> SNAQENQVHIWAVGGCGGEIGSAFEGEVAKGLHSMTYVDTSRANLRDSTLGDDHIYIFKDAAGRELDGSGKKRDENAELICSQIPGILNKHTPGKFNIVVFSLSGGSGSVAGPALVANLLERGERVVCCIVASFDDERQTINADRTFKGLMAAAEGLKRPVIVSYHMNGENGKSEQDVNLDVQVVISQLCVLFSGENRRLDSADLENFLNHPRVTGLEPTITELNTFMGYEWTKENDSPIAFCTLYPKDATKVMGVSAIYSCDGFVPESSPIREATSFVLSTDRLGGIIKQIADEA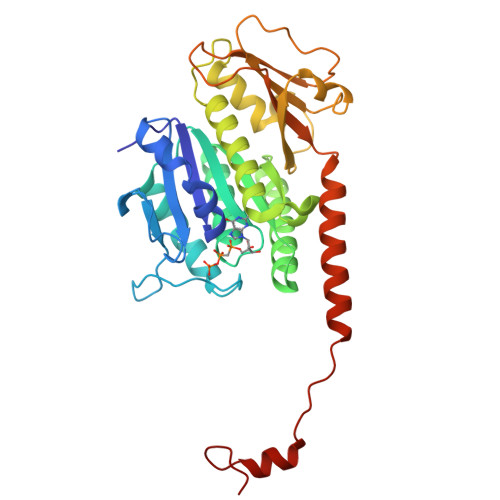KRYIEHRNARQQAPKVGDETVAEAKNSGFLLF However, we were able to solve the first VRR-Nuc domain structures using single-domain proteins derived from three bacteria and bacteriophage as surrogates: Psychrobacter (psNUC); Streptococcus equi bacteriophage P9 (stNUC); and Salmonella enteritidis typing phage 3 (saNUC). Crystal structures of three representatives show that they structurally resemble Holliday junction resolvases (HJRs), are dimeric in solution, and are able to cleave symmetric four-way junctions. DALI searches show that the structures with greatest similarity to the VRR-Nuc domains are all Holliday-junction-resolving enzymes exemplified by Hjc. As dimers, bacterial VRR-Nuc domains have two active sites and a DNA-binding surface with 2-fold symmetry that are well suited to the recognition and symmetrical, bilateral cleavage of Holliday junctions.

stNUC was solved by single-wavelength anomalous diffraction (SAD) methods on crystals of selenomethione-substituted protein and refined against native 1.3 Å resolution data. One molecule is present per asymmetric unit (AU) and comprises a central four-stranded β sheet surrounded by three α helices in a αβββαβα topology. The protein crystallized as a dimer with monomers related by a crystallographic 2-fold axis and interacting through a substantial hydrophobic interface formed by the central β sheets of opposing molecules and bounded on either side by the α2 helix from each partner. Electrostatic surface representations highlight the position of the negatively charged active sites on each monomer, which bind a single magnesium ion in a geometry that is distorted from a classical octahedral arrangement toward a square pyramidal configuration. K47 is presumably involved in positioning the catalytic water molecule as would be expected from homology with other members of the restriction endonuclease-like superfamily (Knizewski et al., 2007). PsNUC bound a four-way DNA junction stoichiometrically with an affinity indicative of a subnanomolar equilibrium dissociation constant (KD) typical of HJRs (∼1 nM; White et al., 1997) whereas stNUC bound the junction over 100 times more weakly (KD = 200 nM). Nevertheless, in both cases, the binding was structure-selective, with psNUC forming weaker complexes with a 5′ flap and a nicked three-way junction and stNUC binding the four-way junction only. stNUC and saNUC exhibited weaker nuclease activity against the Jbm5 HJ substrate, detectable only at protein concentrations above 1 μM and with increased reaction times. Under these conditions, stNUC showed robust activity, whereas cleavage by saNUC was much reduced. In both cases, we observed a range of symmetrical cleavage sites within or close to the homologous core of the junction as well as some nonsymmetrical sites away from the branchpoint. stNUC also selectively cleaved a nicked three-way junction (RF) and a 3′ flap structure (3′F) 2 bp 3′ to the branchpoint.

> GSMRTEKDIENYLKKKTKGLCLKFTSPGTIGVPDRIVVMNTGTFFVEVKAPGKKPRPSQVAMHKKIKEAGQHVWVVDSYESVDMALKEMENW> KISPIETVPVKLKPGMDGPKVKQWPLTEEKIKALVEICTEMEKEGKISKIGPENPYNTPVFAIKKKDSTKWRKLVDFRELNKRTQDFWEVQLGIPHPAGLKKKKSVTVLDVGDAYFSVPLDEDFRKYTAFTIPSINNETPGIRYQYNVLPQGWKGSPAIFQSSMTKILEPFRKQNPDIVIYQYMDDLYVGSDLEIGQHRTKIEELRQHLLRWGLTTPDKKHQKEPPFLWMGYELHPDK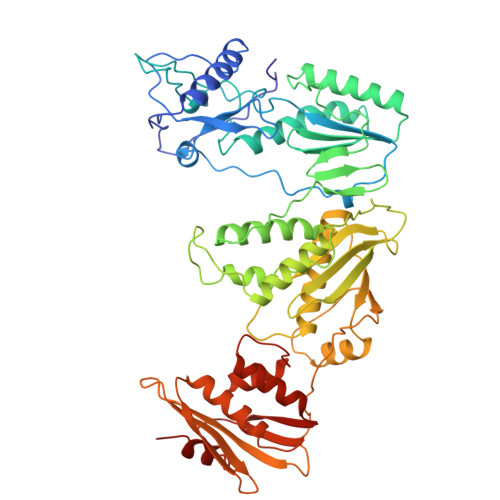WTVQPIVLPEKDSWTVNDICKLVGKLNWASQIYPGIKVRQLCKLLRGTKALTEVIPLTEEAELELAENREILKEPVHGVYYDPSKDLIAEIQKQGQGQWTYQIYQEPFKNLKTGKYARMRGAHTNDVKQLTEAVQKITTESIVIWGKTPKFKLPIQKETWETWWTEYWQATWIPEWEFVNTPPLVKLWYQLEKEPIVGAETFYVDGAANRETKLGKAGYVTNKGRQKVVPLTDTTNQKTQLQAIYLALQDSGLEVNIVTDSQYALGIIQAQPDESESELVNQIIEQLIKKEKVYLAWVPAHKGIGGNEQVDKLVSA>[2x]MERMDCIFCKIANGEIPSTKVYEDDRVLAFNDLNPVAPYHILVV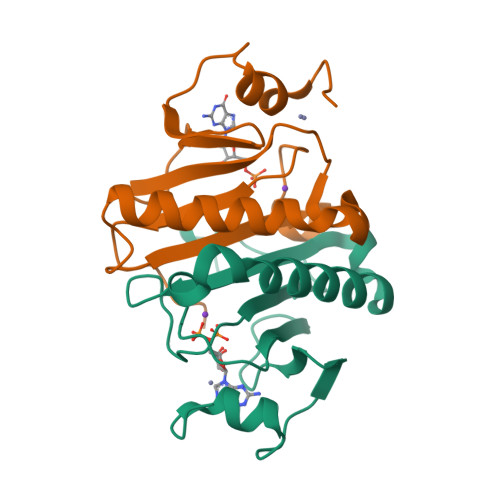PKKHYDSLIDIPDKEMDIVSHIHVVINKIAKEKGFDQTGFRVINNCGSDGGQEVKHLHYHILAGKKLPNYEAGQN The protein that gives the process its name, Clathrin, is a triskelion composed of three heavy chains (Clathrin Heavy Chain, Chc) that provide the structural backbone of the lattice, further stabilized and regulated by three light chains (Clathrin Light Chain, Clc). The proximal domain specifically interacts with Clcs, whereas, the N-terminal domain (NTD) of Chc, which adopts a WD40 beta-propeller structure, is pivotal for interactions with various adaptor proteins (APs). To investigate the existence of binding sites present in Clathrin NTD, we crystallized the N-terminal domain of Chc with different peptides derived from adaptor proteins containing CBMs. All our structures show that each peptide binds to three different binding pockets (Clathrin, Arrestin and W-box).

Crystal structure of Chc-NTD (displayed as a grey cartoon) bound to CBMs from Ent1 (1.75 Å, red), Ent2 (1.74 Å, yellow), Ent5 (Ent5.1 LIDL motif, 2.01 Å, green), Apl2.1 (Apl2.1 LLDLF motif, 2.75 Å, blue) and Yap1801 (1.95 Å, grey). The NTD structures for all complexes are very similar with Cɑ RMSDs between 0.36 Å and 0.64 Å (compared to Ent2 as reference between residues 5 and 336: Ent1 = 0.64 Å, Ent5 = 0.57 Å, YAP1801 = 0.36 Å and APL2 = 0.53 Å) with the exception of the structure in complex with Apl2 that shows the formation of a terminal helix (residues 337–363), transitioning from a helix-turn-helix configuration to an extended, straight helix. An unexpected structural difference observed for the crystal complex with Apl2.1 is the formation of a terminal helix, enabled by the dimerization of two NTD molecules. The presence of alternative secondary structure elements could introduce differences in the overall stability of the Chc complexes or could suggest a mechanism for transmitting signals from the N-terminal domain to the Chc repeat region. Additionally, K98 interacts with position −2 of the motif as observed in the Ent5.1, Apl2.1 and Yap1801 complexes. Concurrently, K326 forms hydrogen bonds with the peptide backbone at positions +2, +4 and +1 for the Ent5.1, Apl2.1 and Yap1801 complexes. Water-mediated interactions are also observed in the W-box between the NTD backbone (L24, D25 and V309) and the peptide at position +3, for both Ent1 and Ent2. However, Apl2.1 and Yap1801 do not show density compatible with water molecules near the binding sites. In addition, the substitution of Ile (from the LIDL motif) for Leu further reduces the binding affinity of Apl2.1 (residues 718-726) for NTD (KDApp ≅ 245 µM).

>GAMAMSDLPIEFTELVDLMSLGISPQFLDFRSTTFESDHFVTVRETKDGTNSVAIVDLAKGNEVTRKNMGGDSAIMHPSQMVISVRANGTIVQIFNLETKSKLKSFTLDEPVIFWRWLSETTLGFVTARSILTSNVFDGNVNAKPQLLTLRHANLNNTQIINFVANKNLDWFAVVGILQENGRIAGRIQLFSKQRNISQAIDGHVAIFTNILLEGNGSTPVQVFVTGNRNATTGAGELRIIEIDHDASLPSQYQKETTDIFFPPDATNDFPIAVQVSEKYGIIYLLTKYGFIHLYELETGTNLFVNRITAESVFTAAPYNHENGIACINKKGQVLAVEISTSQIVPYILNKLSNVALALIVATRGGLPGADDL[2x];>SQDLLDLF[5x]>MGHHHHHHMIEWIIRRSVANRFLVLMGALFLSIWGTWTIINTPVDALPDLSDVQVIIKTSYPGQAPQIVENQVTYPLTTTMLSVPGAKTVRGFSQFGDSYVYVIFEDGTDPYWARSRVLEYLNQVQGKLPAGVSAELGPD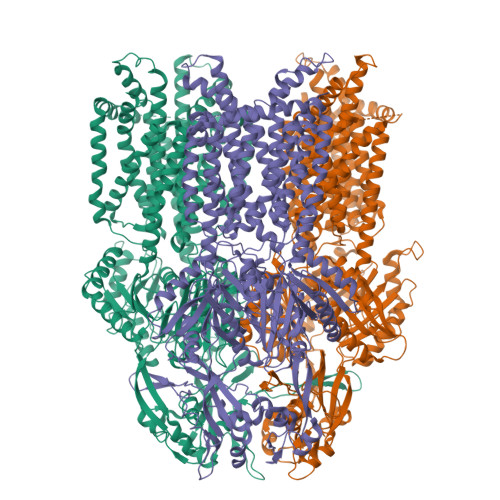ATGVGWIYEYALVDRSGKHDLADLRSLQDWFLKYELKTIPDVAEVASVGGVVKEYQVVIDPQRLAQYGISLAEVKSALDASNQEAGGSSIELAEAEYMVRASGYLQTLDDFNHIVLKASENGVPVYLRDVAKVQIGPEMRRGIAELNGEGEVAGGVVILRSGKNAREVIAAVKDKLETLKSSLPEGVEIVTTYDRSQLIDRAIDNLSGKLLEEFIVVAVVCALFLWHVRSALVAIISLPLGLCIAFIVMHFQGLNANIMSLGGIAIAVGAMVDAAIVMIENAHKRLEEWQHQHPDATLDNKTRWQVITDASVEVGPALFISLLIITLSFIPIFTLEGQEGRLFGPLAFTKTYAMAGAALLAIVVIPILMGYWIRGKIPPESSNPLNRFLIRVYHPLLLKVLHWPKTTLLVAALSVLTVLWPLNKVGGEFLPQINEGDLLYMPSTLPGISAAEAASMLQKTDKLIMSVPEVARVFGKTGKAETATDSAPLEMVETTIQLKPQEQWRPGMTMDKIIEELDNTVRLPGLANLWVPPIRNRIDMLSTGIKSPIGIKVSGTVLADIDAMAEQIEEVARTVPGVASALAERLEGGRYINVEINREKAARYGMTVADVQLFVTSAVGGAMVGETVEGIARYPINLRYPQSWRDSPQALRQLPILTPMKQQITLADVADIKVSTGPSMLKTENARPTSWIYIDARDRDMVSVVHDLQKAIAEKVQLKPGTSVAFSGQFELLERANHKLKLMVPMTLMIIFVLLYLAFRRVGEALLIISSVPFALVGGIWLLWWMGFHLSVATGTGFIALAGVAAEFGVVMLMYLRHAIEAVPSLNNPQTFSEQKLDEALYHGAVLRVRPKAMTVAVIIAGLLPILWGTGAGSEVMSRIAAPMIGGMITAPLLSLFIIPAAYKLMWLHRHRVRK[3x]> GPLGSPLLQQIHNITSFIRQAKAAGRMDEVRTLQENL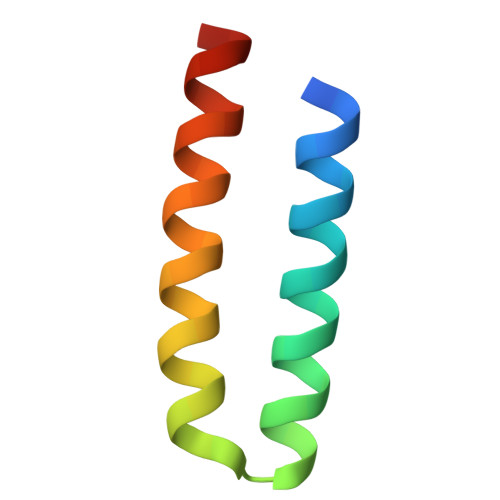RQLQDEYDQQQTEK>VGPKTGEENQVLVPNLNPTPENLEVVGDGFKITSSINLVGEEEADENAVNALREFLTANNIEINSENDPNSTTLIIGEVDDDIPELDEALNGTTAENLKEEGYALVSNDGKIAIEGKDGDGTFYGVQTFKQLVKESNIPEVNITDYPTVSARGIVEGFYGTPWTHQDRLDQIKFYGENKLNTYIYAPKDDPYHREKWREPYPESEMQRMQELINASAENKVDFVFGISPGIDIRFDGDAGEEDFNHLITKAESLYDMGVRSFAIYWDNIQDKSAAKHAQVLN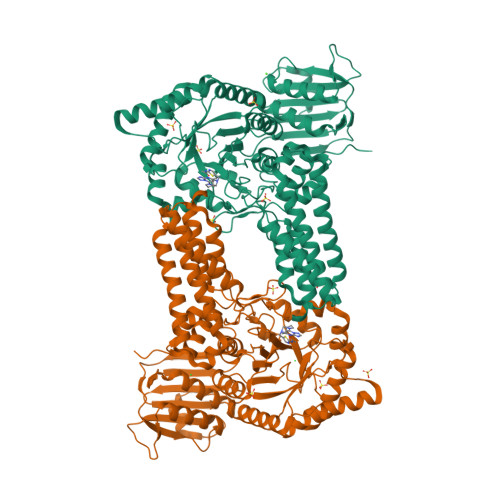RFNEEFVKAKGDVKPLITCPTEYDTGAMVSNGQPRAYTRIFAETVDPSIEVMWTGPGVVTNEIPLSDAQLISGIYDRNMAVWWNYPVTDYFKGKLALGPMHGLDKGLNQYVDFFTVNPMEHAELSKISIHTAADYSWNMDNYDYDKAWNRAIDMLYGDLAEDMKVFANHSTRMDNKTWAKSGREDAPELRAKMDELWNKLSSKEDASALIEELYGEFARMEEACNNLKANLPEVALEECSRQLDELITLAQGDKASLDMIVAQLNEDTEAYESAKEIAQNKLNTALSSFAVISEKVAQSFIQEALSFDLTLI[6x]The second and third steps of the histidine biosynthetic pathway (HBP) in plants are catalyzed by a bifunctional enzyme–HISN2. The enzyme consists of two distinct domains, active respectively as a phosphoribosyl-AMP cyclohydrolase (PRA-CH) and phosphoribosyl-ATP pyrophosphatase (PRA-PH). In this work, we obtained crystal structures of HISN2 enzyme from Medicago truncatula (MtHISN2) and described its architecture and interactions with AMP. The enzyme dimer is formed by two mutually swapped polypeptide chains, forming a bilobial protein—each domain forms one lobe.

The unliganded protein (with metals) crystallized in the C2 space group with two protein chains in the asymmetric unit (ASU). The X-ray structure of MtHISN2 was solved by experimental phasing using single-wavelength anomalous dispersion (SAD) on zinc cations bound to the protein. However, the MtHISN2 crystals could only be grown in the presence of a low concentration of Zn2+ in addition to Mg2+. There are two unique MBSs in the PRA-PH domain. MBS1 contains Zn2+ coordinated by two carboxyl oxygen atoms of Glu220 and one carboxyl oxygen of Glu217. In MBS2, Zn2+ is tetrahedrally coordinated by carboxylic groups of Glu214, Glu234, Asp237, and a water molecule. The MBS3 is formed by the carboxylic groups of Asp125*, Asp127*, Asp129* and by two water molecules in a shape of a trigonal bipyramid. In the next site, MBS4, Zn2+ is coordinated tetrahedrally by two water molecules and Nε of His143 and by the thiol of Cys126*. Lastly, Zn2+ bound in the MBS5 is coordinated by thiols of Cys126*, Cys142, and Cys149. A metal cation (MBS4) may play a role in priming His143; in the unliganded MtHISN2 structure, His143 does not bind a water molecule but instead is in the MBS4 coordination sphere.

>SNAVDSLLDSVKWDNKGLAVAIAQNVDTGAILMQGFANREAVATTISSRKATFYSRSRSSLWTKGETSNNFINVHDVFLDCDRDSIIYLGKPDGPTCHTGAETCYYTPVFDLLKEEEVEGNKLALTSLYALESTISQRKAEVVEENGKPSWTKRLLLNDKLLCSKIREEANELCETLENNEDKSRTASEMADVLYHAMVLLALKDVKVEEVLQVLRQRFSKSGIEEKRSRPTQKSVEN[2x]2,5-DINITROPHENOL | C6 H4 N2 O5 | 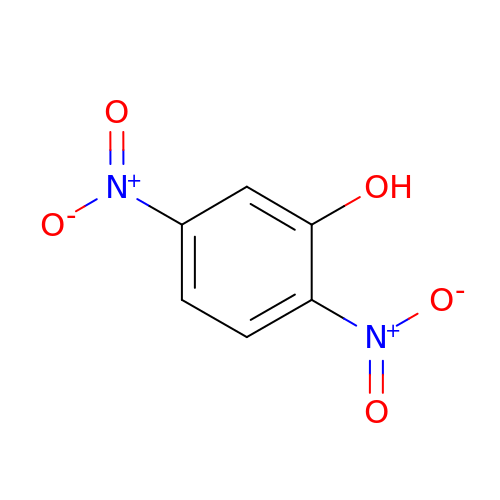UWEZBKLLMKVIPI-UHFFFAOYSA-N>GHMEQTARAIFRFVPRHEDELELEVDDPLLVELQAEDYWYEAYNMRTGARGVFPAYYAIEVTK[2x]

Aromatic residues cluster in the core of folded proteins, where they stabilize the structure through multiple interactions. NMR studies in the 1970s demonstrated that aromatic side chains can undergo ring flips—that is, 180° rotations of the χ2 dihedral angle (Cβ–Cγ axis)—even when engaged in stabilizing interactions in the hydrophobic core. Here we capture ring flipping events of a buried tyrosine residue in the SH3 domain of the JNK-interacting protein 1 (JIP1). Our data therefore suggest that the conformation of the aromatic ring at position 526 is determined by steric interactions dictated by the size of the surrounding amino acids.

Accordingly, we designed four different mutants of JIP1-SH3 (H493A, V517A, V517L and A541L) and obtained their high-resolution structures by X-ray crystallography. Of note, three mutants (H493A, V517A and A541L) induce a staggered conformation of Y526, with χ2 dihedral angles ranging from −41° to −75°, whereas V517L shows an eclipsed conformation of Y526 and an almost identical structure to the wild-type protein. The H493A and V517A variants show almost identical crystal structures and for a subset of residues, the chemical shifts of which are unaffected by the mutations, the resonances of the two variants fall on a straight line together with the resonances of the wild-type protein. This suggests that they are in fast–intermediate exchange between two conformations represented by the crystal structures of the wild-type protein and of the H493A/V517A variants. In agreement with this, both variants show line broadening and chemical exchange contributions as detected by 15N and 1HN relaxation dispersion. Analysis of these data shows that the structural features of the minor state of the wild-type protein are captured by the H493A/V517A crystal structures, as shown by the excellent agreement between the ΔδCPMG values for the wild-type protein and the two variants. In addition, the analysis yields exchange rates between the staggered (canonical β-strand) and the eclipsed (classic β-bulge) conformation of kEX = 2,830 ± 70 s−1 (H493A) and kEX = 6,800 ± 300 s−1 (V517A), compared to kEX = 2,600 ± 70 s−1 determined for the wild-type protein. Finally, the observable chemical shifts of the two variants, in conjunction with analysis of the relaxation dispersion data (Supplementary Discussion), show that the H493A mutation slightly stabilizes the minor state relatively to the major state, whereas the V517A mutation almost inverts the relative populations of the major and minor states.> MITIITQDQLKTSPSVREDGRAFDELRPLKIEAGILERADGSSYLEFGGNKILVAVYGPREAQIRKLQRPDRAVIRCRYNMAPFSVEERKRPGPDRRSVEISKITAEALRPALILEKFPRSVIDVFIEVLEAEGGTRCAGITAASVALADAGIPMRDMVVACAAGKVGDQVVLDLSEEEDKEGQADVPVAIL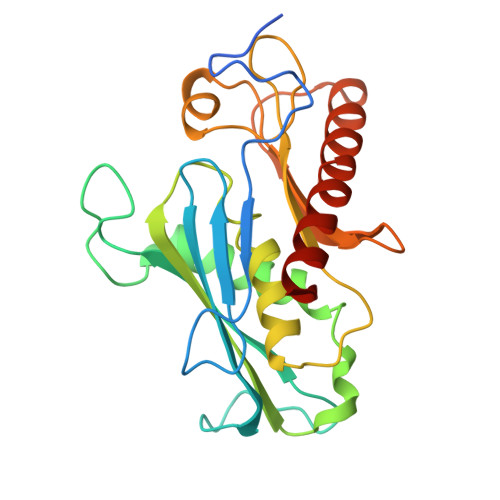PRTREITLLQSDGNLTPEEFERALDLAVEGCLRIHEVQKEALRKRYGE> SHMTNLQTFELPTEVTGCAADISLGRALIQAWQKDGIFQIKTDSEQDRKTQEAMAASKQFCKEPLTFKSSCVSDLTYSGYVASGEEVTAGKPDFPEIFTVCKDLSVGDQRVKAGWPCHGPVPWPNNTYQKSMKTFMEELGLAGERLLKLTALGFELPINTFTDLTRDGWHHMRVLRFPPQTSTLSRGIGAHTDYGLLVIAAQDDVGGLYIRPPVEGEKRNRNWLPGESSAGMFEHDEPWTFVTPTPGVWTVFPGDILQFMTGGQLLSTPHKVKLNTRERFACAYFHEPNFEASAYPLFEPSANERIHYGEHFTNMFMRCYPDRITTQRINKENRLAHLEDLKKYSDTRATGS

The ethylene-forming enzyme (EFE) is an Fe(II), 2-oxoglutarate (2OG), and l-arginine (l-Arg)-dependent oxygenase that either forms ethylene and three CO2/bicarbonate from 2OG or couples the decarboxylation of 2OG to C5 hydroxylation of l-Arg. l-Arg binds with C5 toward the metal center, causing 2OG to change from monodentate to chelate metal interaction and OD1 to OD2 switch of D191 metal coordination. The best characterized EFE is that from the Pseudomonas savastanoi (formerly Pseudomonas syringae) pv phaseolicola strain PK2, for which several crystal structures have been reported. This enzyme binds mononuclear Fe(II) using three side chains (H189, D191, and H268) with three water molecules completing the six-coordinate geometry. Here, we extend our understanding of EFE catalysis by carrying out biochemical, structural, and computational studies of the enzyme in complex with a substrate analogue and using two enzyme variants. In combination, the results presented here are compatible with the currently proposed enzyme mechanism,4−8 emphasize the necessity for OD2 of D191 to coordinate the metal, and highlight the importance of the second coordination sphere and longer range interactions in promoting EFE activity.

First, we consider the binding of l-canavanine, a chemical analogue of l-Arg in which the C5 methylene group is replaced by an oxygen atom. The EFE cannot transform this analogue into guanidine and P5C, but we also showed that the l-canavanine-bound enzyme fails to induce ethylene generation. To understand this lack of reactivity, we used anaerobic ultraviolet–visible (UV–vis) spectroscopy to examine the effect of l-canavanine on the metal-to-ligand charge-transfer (MLCT) transitions of EFE·Fe(II)·2OG and determined the structure of the EFE·Mn(II)·2OG·l-canavanine complex. l-Canavanine binds to the EFE with its O5 atom pointing away from the metal center, whereas C5 of l-Arg points toward the iron atom, consistent with the ability of the enzyme to react with only the latter compound. Anaerobic UV–vis spectroscopy of EFE·Fe(II)·2OG·l-canavanine and structural studies of EFE·Mn(II)·2OG·l-canavanine confirm that binding of the substrate analogue leads to bidentate coordination of 2OG to Fe(II). Critical insights into why the l-canavanine-bound enzyme is ineffective for ethylene generation were obtained from the crystal structure of EFE·Mn(II)·2OG·l-canavanine that revealed that OD1 of D191 coordinated the metal instead of the catalytically productive OD2 coordination noted for bound l-Arg. The ineffective l-Arg analogue l-canavanine binds to the EFE with O5 pointing away from the metal center while promoting chelate formation by 2OG but fails to switch the D191 metal coordination from OD1 to OD2. Congruent with the structural results, MD simulations predict that the most favored l-canavanine conformation in the EFE·Fe(III)·OO•–·2OG·l-canavanine complex has its O5 pointed away from the metal center and facing toward E84.3-fluoro-N-hydroxy-4-[(methyl{[(3s,5s,7s)-tricyclo[3.3.1.1~3,7~]decan-1-yl]methyl}amino)methyl]benzamide 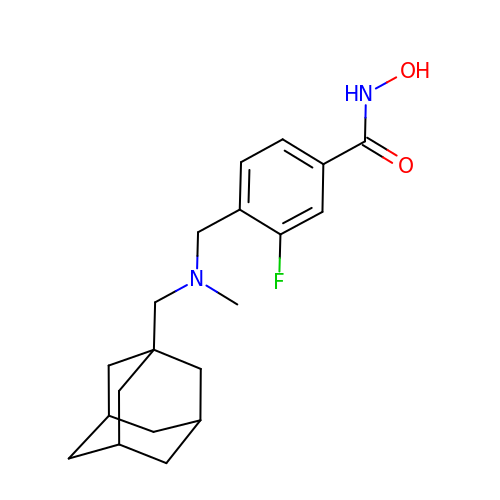| C20 H27 F N2 O2 | IGZQZELTOHAHNW-PVGDPBLGSA-N N-(phosphonomethyl)glycine | C3 H8 N O5 P | 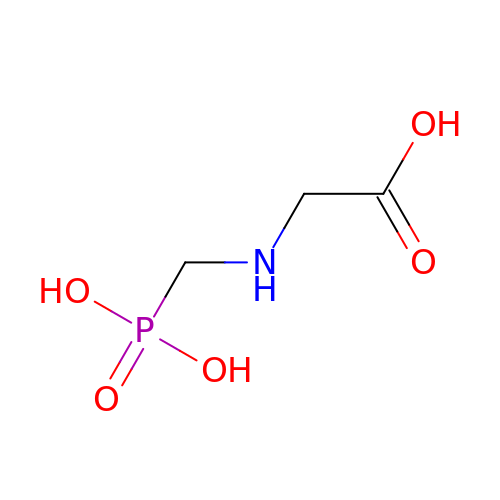XDDAORKBJWWYJS-UHFFFAOYSA-N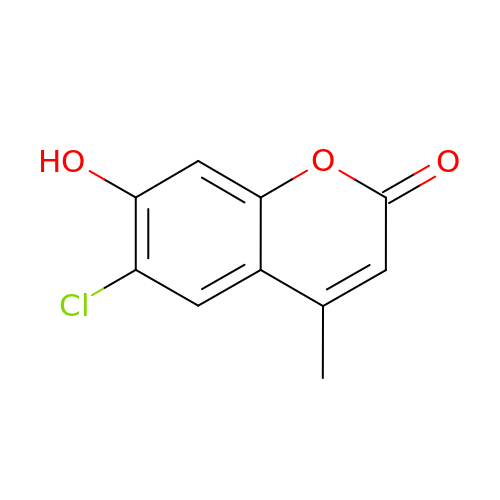6-chloro-7-hydroxy-4-methyl-2H-chromen-2-one | C10 H7 Cl O3 | JTXAGHXRIBLWES-UHFFFAOYSA-N>TLFVEYIGYPLFSGVKFSDVPINPHITKFQFVLSFAVDYTASSPHTSTNGKFNVFWDSSILGPDQISAIKSSHPNVRVAVSLGGASVGSNTVQFQAASVDSWVSNAVTSLTRIIQRYNLDGIDIDYEHFQNTDKNTFAECIGRLITTLKKNGVISFASIS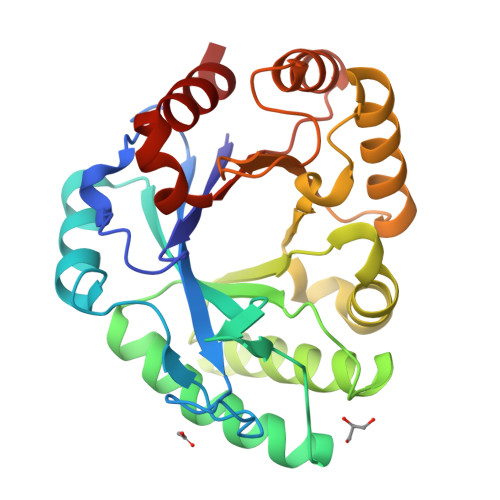PFPSVDEYYLALFNEYKNAINHINYQFKAYDSSTSVDKFLGYYNNAASKYKGGNVLISFSTGPHPGGLPVDKGFFDAATSLKNKGKLHGIAVWTADTSKSSDFRYEEEAQAFLVS[2x]Focal Adhesion Kinase (FAK) is a 125 kDa non-receptor tyrosine kinase that has multiple implications in cancer cell signaling, invasion, proliferation, and metastasis. Activation of FAK occurs not only through autophosphorylation of key residue tyrosine 397 (Y397) by FAK itself via the kinase enzyme, but also through transphosphorylation by receptor tyrosine kinases which can bind to the FAK N-terminal FERM domain directly. The proto-oncogene Src directly binds to FAK through its SH2 and SH3 domains at phosphorylated FAK Y397 and a proline-rich region in the FERM-Kinase linker, respectively. FAK also functions as an intracellular scaffolding protein through its FERM domain and C-terminal FAT domain regions where FAK forms multiple protein-protein interactions to connect oncogenic signaling pathways.

Here, we report an x-ray crystal structure of the avian FAK FERM domain at a higher resolution (1.97 Å) than previously reported, elucidating new structural features of the FERM-Kinase linker segment that impact the druggability of the Y397 region. The protein crystallized in the orthorhombic space group P 212121 with two molecules per asymmetric unit. The overall conformation of the FERM molecule displays strong structural similarity with other FERM domains of ERM family members ezrin, radixin, and moesin, consisting of three subdomains (labeled F1, F2, and F3). In this work, we solved the FERM structure at a much higher 1.97 Å resolution and we were able to rebuild the segment (363–375) in this area including the RALPSIP motif. Residues L370 and P371 of the SH3 binding motif from FERM molecule A pack into a pocket formed by residues I359, Y304, E338, M102, and H99 in between the F1 and F3 lobes of the protein. Residues 372–375 of the motif bind along the side of the F1 lobe however visibility of residues 376–390 cannot be determined. In our structure, the Src SH3 binding site makes intramolecular contacts with a pocket in between the FERM F1 and F3 lobes. We speculate that the intramolecular interactions between the Src SH3 binding site and the FERM F1/F3 lobes may be an “autoinhibited” conformation that prevents binding of Src to FAK and therefore the full activation of FAK by phosphorylation of Y576, Y577, Y861, and Y925. Upon further examination in PyMOL we noticed a significant difference in electron density of key activation residue Y397 and surrounding residues in the FERM-kinase linker as well as residues in the F1 lobe proximal to Y397. Computational prediction of this pocket in our structure suggested that the Y397 region has poor druggable characteristics, contrasting previous reports.

>[2x]GSMGAMERVLKVFHYFENSSEPTTWASIIRHGDATDVRGIIQKIVDCHKVKNVACYGLRLSHLQSEEVHWLHLDMGVSNVREKFELAHPPEEWKYELRIRYLPKGFLNQFTEDKPTLNFFYQQVKNDYMLEIADQVDQEIALKLGCLEIRRSYGEMRGNALEKKSNYEVLEKDVGLRRFFPKSLLDSVKAKTLRKLIQQTFRQFANLNREESILKFFEILSPVYRFDKECFKCALGSSWIISVELAIGPEEGISYLTDKGANPTHLADFNQVQTIQYSNSEDKDRKGMLQLKIAGAPEPLTVTAPSLTIAENMADLIDGYCRLVNGATQSFIIRPQKEGERALPSIPKLANNEKQGVRSHTVSVSETDDYAEIIDEED>[2x]MPVVECDIQTARAALADAGASFSDGNSEHELWHADLGDAHAVAYADKLVVQGGSPTDITAVVQP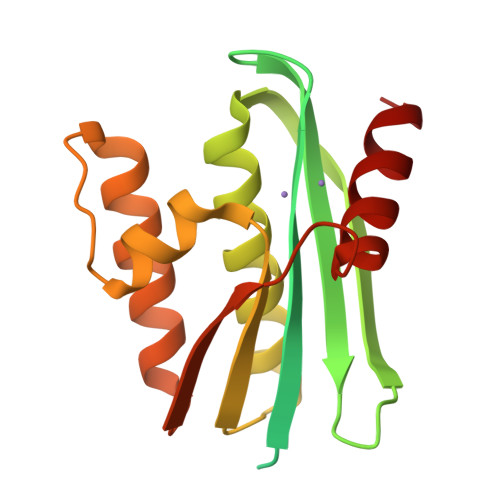DRGGRVHAYFDGASRGNPGPAAVGWVLVSGDGGIVAEGGDTIGRATNNQAEYDALIAALEAAADFGFDDIELRGDSQLVEKQLTGAWDTNDPDLRRKRVRARELLTGFDDWSITHVPRATNERADALANEALDDA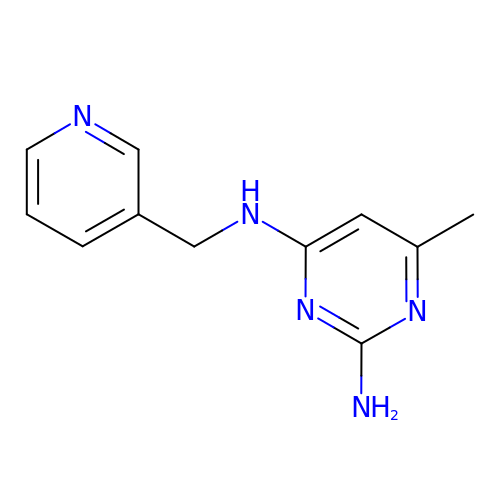6-methyl-N~4~-[(pyridin-3-yl)methyl]pyrimidine-2,4-diamine | C11 H13 N5 | DSSCXCDTPABWJX-UHFFFAOYSA-N SPOUT1, also known as CENP-32 or C9ORF114, contains a putative SpoU-TrmD (SPOUT) RNA methyltransferase (MTase) domain. SPOUT1/CENP-32 localized to mitotic spindles and kinetochores, and its depletion by siRNA resulted in unusual centrosome detachment from the mitotic spindle poles, delayed anaphase onset, and chromosome segregation errors. Structural analysis confirmed that SPOUT1/CENP-32 is a SPOUT MTase with a trefoil knot fold consisting of parallel six stranded β-sheets sandwiched between two layers of α-helices that promote dimerization of the protein. Our SPOUT1/CENP-32 structures also reveal that SPOUT1/CENP-32 dimerizes via a helical segment in the catalytic domain that packs almost perpendicularly against an equivalent segment from its dimeric counterpart.

SPOUT MTases use S-adenosyl-L-methionine (SAM) as the methyl group donor for the methyltransferase reaction. To determine whether SPOUT1/CENP-32 can also bind the cofactor, SAM, and to gain further structural insights into the substrate binding site, we soaked the SPOUT1/CENP-32 crystals in a cryo-protectant solution containing a molar excess of SAM prior to freezing the crystals for X-ray data collection. These crystals diffracted X-rays beyond 2.62 Å. The SAM-bound structure of SPOUT1/CENP-32 was determined using molecular replacement. The difference electron density map calculated for the refined model showed a well-defined electron density for the bound SAM. The mode of SAM binding is similar to that of SAH, with a methyl group pointing out of the deep cofactor binding pocket. The binding of SAH and SAM is similar. E Close-up of the electrostatic surface potential of SPOUT1/CENP-32 71-376 bound to SAM showing the deep pocket formed by the trefoil knot.

> MRPYTLSVALPGSILDNAQSPELRTYLAGQIARACAIFCVDEIVVFDEEGQDAKTVEGEFTGVGKKGQACVQLARILQYLECPQYLRKAFFPKHQDLQFAGLLNPLDSPHHMRQDEESEFREGIVVDRPTRPGHGSFVNCGMKKEVKIDKNLEPGLRVTVRLNQQQHPDCKTYHGKVVSSQDPRTKAGLYWGYTVRLASCLSAVFAEAPFQDGYDLTIGTSERGSDVASAQLPNFRHALVVFGGLQGLEAGADADPNLEVAEPSVLFDLYVNTCPGQGSRTIRTEEAILISLAALQPGLIQAGARHT> MSTPARKRL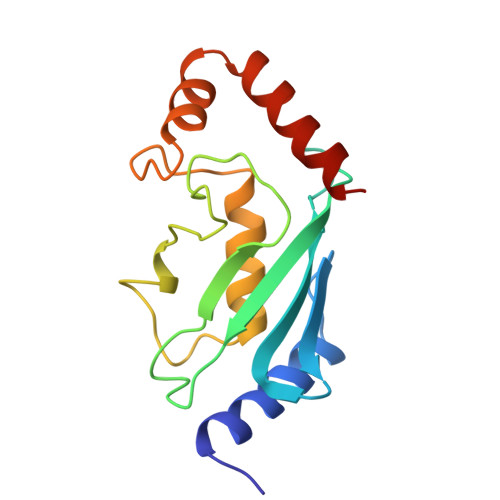MRDFKRLQQDPPAGISGAPQDNNIMLWNAVIFGPDDTPWDGGTFKLSLQFSEDYPNKPPTVRFVSRMFHPNIYADGSICLDILQNQWSPIYDVAAILTSIQSLLCDPNPNSPANSEAARMYSESKREYNRRVRDVVEQSWTAD> IESIIKTATDTVKSEINAELGVVPSLNAVETGATSNTEPEEAIQTRTVINQHGVSETLVENFLSRAALVSKRSFEYKDHTSSTARADKNFFKWTINTRSFVQLRRKLELFTYLRFDAEITILTTVAVNGSGNNTYVGLPDLTLQAMFVPTGALTPEKQDSFHWQSGSNASVFFKISDPPARITIPFMCINSAYSVFYDGFAGFEKNGLYGINPADTIGNLCVRIVNEHQPVGFTVTVRVYMKPKHIKAWAPRPPRTLPYMSIANANYKGKERAPNALSAIIGNRDSVKTMPHNIVNT;> GVPTYLLPGSGQFLTTDDHSSAPALPCFNPTPEMHIPGQVRNMLEVVQVESMMEINNTESAVGMERLKVDISALTDVDQLLFNIPLDIQLDGPLRNTLVGNISRYYTHWSGS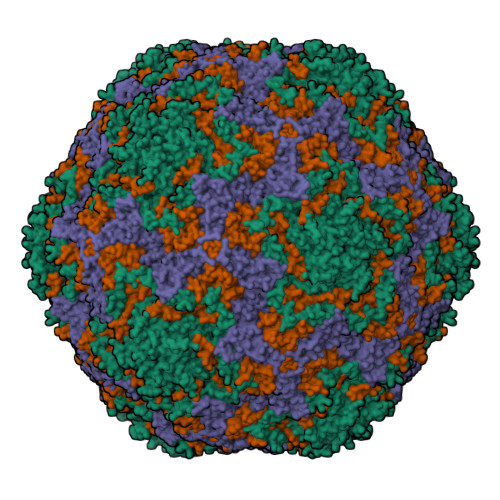LEMTFMFCGSFMAAGKLILCYTPPGGSCPTTRETAMLGTHIVWDFGLQSSVTLIIPWISGSHYRMFNNDAKSTNANVGYVTCFMQTNLIVPSESSDTCSLIGFIAAKDDFSLRLMRDSPDIGQLDHLHAAEAAYQ;> SPSAEACGYSDRVLQLKLGNSAIVTQEAANYCCAYGEWPNYLPDHEAVAIDKPTQPETATDRFYTLKSVKWETGSTGWWWKLPDALNNIGMFGQNVQHHYLYRSGFLIHVQCNATKFHQGALLVVAIPEHQRGAHNTNTSPGFDDIMKGEEGGTFNHPYVLDDGTSLACATIFPHQWINLRTNNSATIVLPWMNAAPMDFPLRHNQWTLAIIPVVPLGTRTTSSMVPITVSIAPMCCEFNGLRHAITQ;> GAQVTRQQTGTHENANIATNGSHITYNQINFYKDSYAASASKQDFSQDPSKFTEPVVEGLKAGAPVLK>TGFDFNAYMGEKAAAVNRALDASIPADEPPAALHEAMRYALLAGGKRVRPALCLAACAVVGGREAWAMPAAAAVEMVHTMSLVHDDLPCMDDDDLRRGKPTCHVVYGEPIAVLTGDALLSLSFHHMARFDSYPPDIDADKHPARVVRAIGELARCIGSEGLVAGQVVDLEMTGSTETVPLERLEYIHLHKTAALLEASVVIGAILGGGSDEQIESLRMYARSIGLLFQVVDDILDVTKSSEELGKTAGKDLASDKTTYPKLLGLEKSREFAEKLLSDAREQLSGFDQETAAPLLHLANYIAYRQN[3x];>SFDLRLYWTSLIADVEAELDAAMPIRTPERIHSAMRYAVLPGAGNEGTAKRAPPVLCVAACELLGAPREAALPAAVALEMLHAASLVHDDLPCFDAAPTRRGRPSTHAAYGTDMAVLAGDALFPLAYTHVIAHTPSPDPVPHAVLLRVLGELARAVGSTGMAAGQFLDLAGATALGEAEVMKVLTKKFGEMAECSAA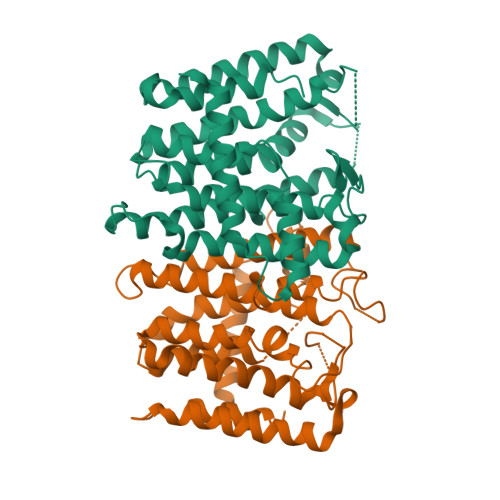CGAMLGGAGPDEEAALRRYGRTIGVLYQLVDDIRSASGNGKMRSNASVLRALGMDRALGIVEELKAQAKMEADRFGDKYGERVLPLYSFVDYAVERGFELQDAATTP[3x]> TVAYIAIGSNLASPLEQVNAAL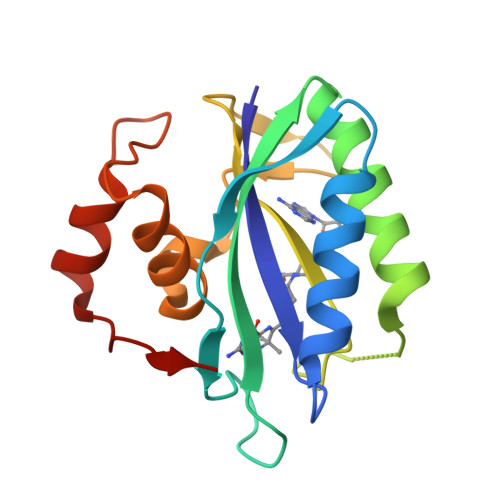KALGDIPESHILTVSSFYRTPPLGPQDQPDYLNAAVALETSLAPEELLNHTQRIELQQGRVRKAERWGPRTLDLDIMLFGNEVINTERLTVPHYDMKNRGFMLWPLFEIAPELVFPDGEMLRQILHTRAFDKLNKW N-{3-[3-(DIMETHYLAMINO)PROPYL]-5-(TRIFLUOROMETHYL)PHENYL}-4-METHYL-3-[(3-PYRIMIDIN-4-YLPYRIDIN-2-YL)AMINO]BENZAMIDE 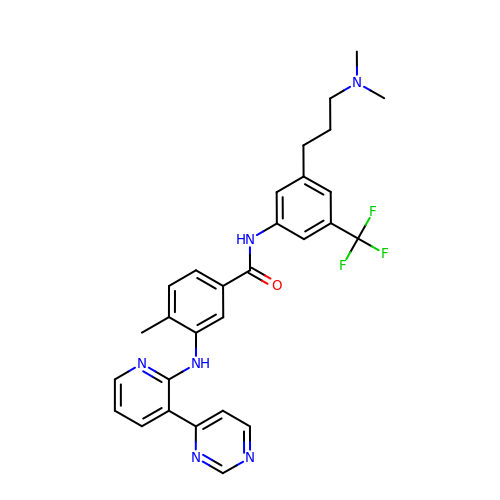| C29 H29 F3 N6 O | OHHGYJBFPVJURR-UHFFFAOYSA-N>VVKRTMTKKFLEEAFAGESMAHMRYLIFAEKAEQEGFPNIAKLFRAIAYAEFVHAKNHFIALGKLGKTPENLQMGIEGETFEVEEMYPVYNKAAEFQGEKEAVRTTHYALEAEKIHAELYRKAKEKAEKGEDIEIKKVYICPICGYTAVDEAPEYCPVCGAPKEKFVVFE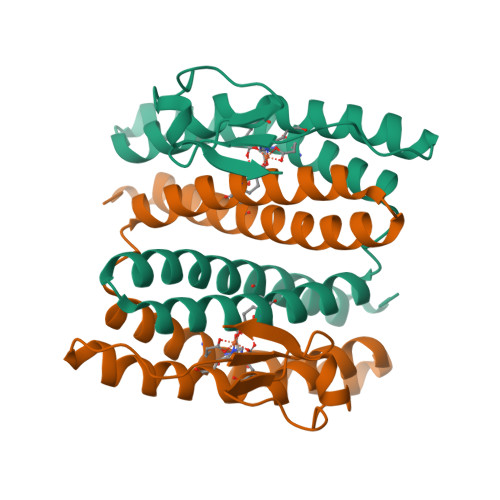[8x]> MSMLKREDWYDLTRTTNWTPKYVTENELFPEEMSGARGISMEAWEKYDEPYKITYPEYVSIQREKDSGAYSIKAALERDGFVDRADPGWVSTMQLHFGAWALEEYAASTAEARMARFAKAPGNRNMATFGMMDENRHGQIQLYFPYANVKRSRKWDWAHKAIHTNEWAAIAARSFFDDMMMTRDSVAVSIMLTFAFETGFTNMQFLGLAADAAEAGDHTFASLISSIQTDESRHAQQGGPSLKILVENGKKDEAQQMVDVAIWRSWKLFSVLTGPIMDYYTPLESRNQSFKEFMLEWIVA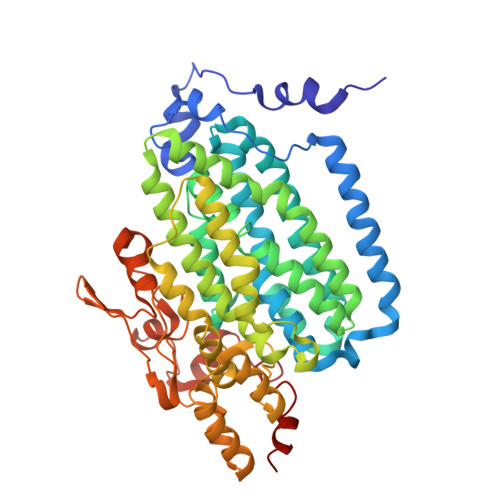QFERQLLDLGLDKPWYWDQFMQDLDETHHGMHLGVWYWRPTVWWDPAAGVSPEEREWLEEKYPGWNDTWGQCWDVITDNLVNGKPELTVPETLPTICNMCNLPIAHTPGNKWNVKDYQLEYEGRLYHFGSEADRWCFQIDPERYKNHTNLVDRFLKGEIQPADLAGALMYMSLEPGVMGDDAHDYEWVKAYQKKTNAA(8S,12S)-15S-HYDROXY-9-OXOPROSTA-10Z,13E-DIEN-1-OIC ACID | C20 H32 O4 | 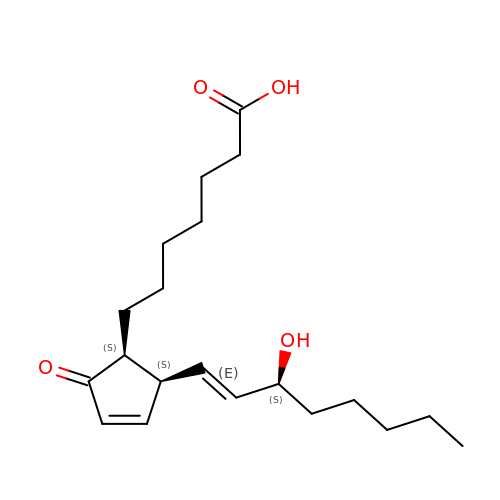BGKHCLZFGPIKKU-DRSVPBQLSA-N> MGSSHHHHHHSSGENLYFQGHMKNVLLIGACGALGRAVANAFAKGKWSI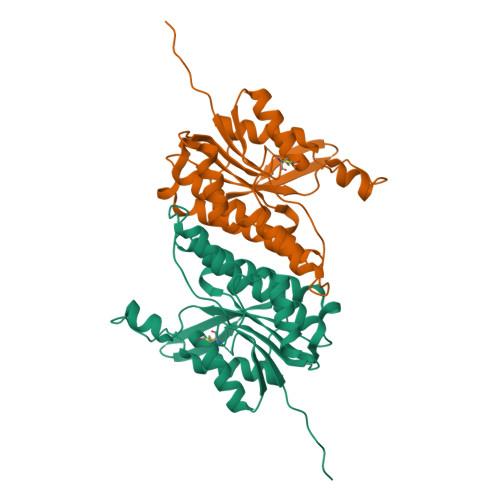ISVDQAAAVQQGDGCGAVNPASSIEELQQAYKSAVTGLKVDAVINVAGGWAGGSVADARTAASTELMLRQSLFSSVAAAHVFSTQGEKDGLLLLTGAAAALSPTPGMIGYGTAKSAVHFLCQSIAADPSVLPTDASVLAILPTILDTPGNRSAMPHADRSTWTSLEDVAQQIVEWSNGSRRPASGSLVKIVTENSKTRFIV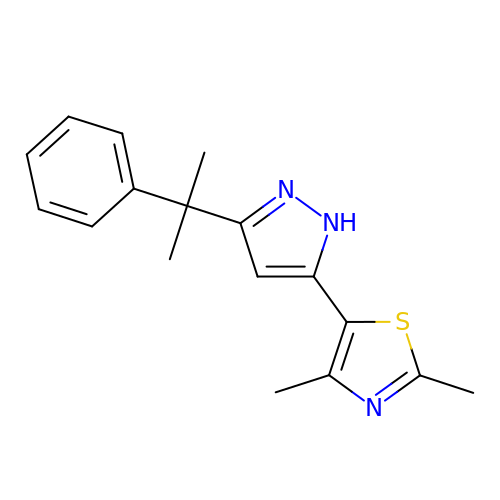2,4-dimethyl-5-[3-(2-phenylpropan-2-yl)-1H-pyrazol-5-yl]-1,3-thiazole | C17 H19 N3 S | FAEGQXWWILYIST-UHFFFAOYSA-N> LPKPGTYYLPWEVSAGQVPDGSTLRTFGRLCLYDMIQSRVTLMAQHGSDQHQVLVCTKLVEPFHAQVGSLYIVLGELQHQQDRGSVVKARVLTCVEGMNLPLL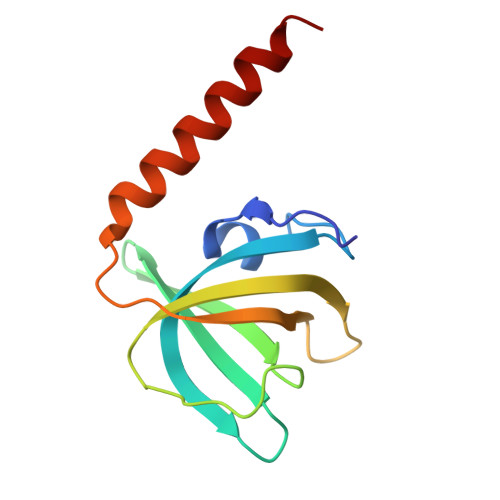EQAIREQRLYKQERGGSQ>[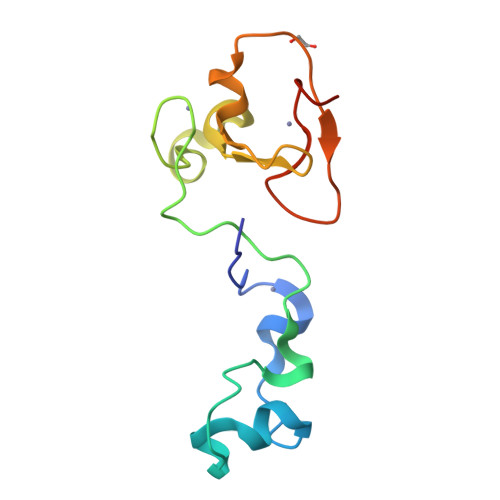2x]SMRRVRCRKCKACVQGECGVCHYCRDMKKFGGPGRMKQSCVLRQCLAPRLPHSVTCSLCGEVDQNEETQDFEKKLMECCICNEIVHPGCLQMDGEGLLNEELPNCWECPKCYQEDSS> MGNIMSASFAPECTDLKTKYDSCFNEWYSEKFLKGKSVENECSKQWYAYTTCVNAALVKQGIKPAL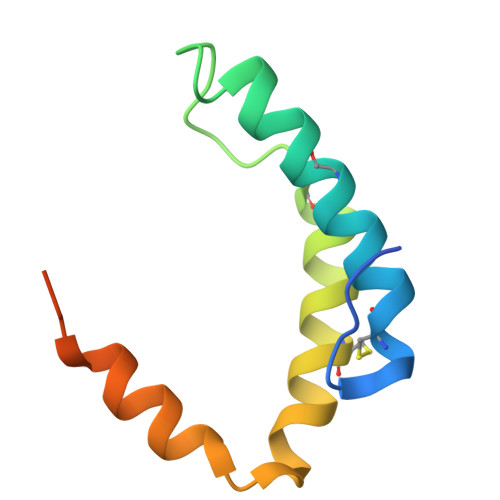DEAREEAPFENGGKLKEVDK>[2x]QDGKTTFEKEGGGGRGPRILENMHE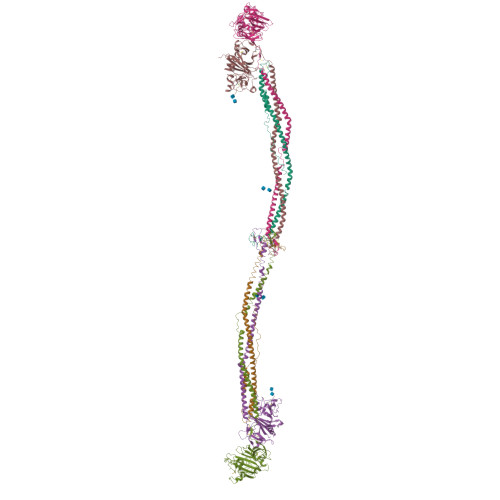SSCKYEKNWPICVDDDWGTKCPSGCRMQGIIDDTDQNYSQRIDNIRQQLADSQNKYKTSNRVIVETINILKPGLEGAQQLDENYGHVSTELRRRIVTLKQRVATQVNRIKALQNSIQEQVVEMKRLEVDIDIKIRACKGSCARSFDYQVDKEGYDNIQKHLTQASSIDMHPDFQTTTLSTLKMRPLKDSNVPEHFKLKPSPEMQAMSAFNNIKQMQVVLERPETDHVAEARGDSSPSHTGKLITSSHRRESPSLVDKTSSASSVHRCTRTVTKKVISGPDGPREEIVEKMVSSDGSDCSHLQGGREGSTYHFSGTGDFHKLDRLLPDLESFFTHDSVSTSSRHSIGSSTSSHVTGAGSSHLGTGGKDKFTDLGEEEEDDFGGLQPSGFAAGSASHSKTVLTSSSSSFNKGGSTFETKSLKTRETSEQLGGVQHDQSAEDTPDFKARSFRPAAMSTRRSYNGKGTQK;>QASVEYDNEEDSPQIDARAHRPLDKRQEAAPTLRPVAPPISGTGYQPRPPKQDKQAMKKGPIIYPDAGGCKHPLDELGVLCPTGCELQTTLLKQEKTVKPVLRDLKDRVAKFSDTSTTMYQYVNMIDNKLVKTQKQRKDNDIILSEYNTEMELHYNYIKDNLDNNIPSSLRVLRAVIDSLHKKIQKLENAIATQTDYCRSPCVASCNIPVVSGRECEDIYRKGGETSEMYIIQPDPFTTPYRVYCDMETDNGGWTLIQNRQDGSVNFGRAWDEYKRGFGNIAKSGGKKYCDTPGEYWLGNDKISQLTKIGPTKVLIEMEDWNGDKVSALYGGFTIHNEGNKYQLSVSNYKGNAGNALMEGASQLYGENRTMTIHNGMYFSTYDRDNDGWLTTDPRKQCSKEDGGGWWYNRCHAANPNGRYYWGGTYSWDMAKHGTDDGIVWMNWKGSWYSMKKMSMKIKPYFPD[2x];>YIATRENCCILDERFGSYCPTTCGIADFFNKYRLTTDGELLEIEGLLQQATNSTGSIEYLIQHIKTIYPSEKQTLPQSIEQLTQKSKKIIEEIIRYENTILAHENTIQQLTDMHIMNSNKITQLKQKIAQLESHCQEPCKDTAEIQETTGRDCQDIANKGARKSGLYFIKPQKAKQSFLVYCEIDTYGNGWTVLQRRLDGSEDFRRNWVQYKEGFGHLSPDDTTEFWLGNEKIHLITTQSTLPYALRIELEDWSGKKGTADYAVFKVGTEEDKYRLTYAYFIGGEAGDAFDGFNFGDDPSDKSYTYHNGMRFSTFDNDNDNFEGNCAEQDGSGWWMNRCHAGHLNGPYYIGGVYSRDTGTNSYDNGIIWATWRDRWYSMKKTTMKIIPFNRLSIDGQQHSGGLKQVGDS[2x];>[2x]GPRP;>[2x]GHRP>MVYKITVRVYQTNPDAFFHPVEKTVWKYANGGTWSITDDQHVLTMGGSGTSGTLRFHADNGESFTATFGVHNYKRWCDIVTNLAADETGMVINQQYYSQKNREEARERQLSNYQVKNAKGRNFQIVYTEAEGNDLHANLIIG[2x]

Sclerotium rolfsii lectin (SRL) is a cell wall-associated developmental–stage specific lectin secreted from the soil–born pathogenic fungus. SRL displays a clear specificity for TF and its substituted glycan structures. In the current study we report two recombinant variants SSR1 and SSR2, generated by the deliberate changes of the amino acids incorporated at particular sites of SRL by the synthetic gene construct method based on the complete amino acid sequence of SRL. Interestingly, SSR1 and SSR2 the two different variants of SRL, differ in their glycan specificity.

In case of SSR2 amino acids at the 1st, 14th, 34th, 113th and 123rd were replaced with Val, Asp, Ser, Gln and Gln, respectively. The crystal structures of SSR1 and SSR2 lectins in their free form were determined at 1.7 Å and 1.6 Å resolution, respectively. Like SRL there are two protein molecules (named mol A and mol B) in the crystallographic asymmetric unit of both variants related by a non-crystallographic two-fold symmetry. The mutations of SSR1 (N14D, E113Q, E123Q) and SSR2 (T1V, N14D, T34S, E113Q, E123Q) were all identified and all atoms of the mutated residues were well defined within the electron density map. A bound MPD molecule was found in both variants at the same place like in SRL while in the SSR2 structure two additional molecules form the crystallization medium were found bound (MPD and a 2-amino-2-hydroxymethyl-propane-1,3 diol). In the structure of SSR2 the mutated residues Val1 and Ser34 are located in strands S1 and S2, respectively. In the SSR2 structure the T1V mutation leads to a shift of the residue by 0.6–1.0 Å (depending on the atoms) while the T34S mutation does not cause any conformational change on this residue. The adoption of this conformation of Asn81 in SSR1 is made possible by a shift of the entire loop encompassing residues 81–86 by 3.0 Å on average, from their positions in the SRL structure. This shift is less profound in the SSR2 structure (1.0 Å on average) and does not lead to a change in the conformation of the side chain of Asn81 which maintains a similar conformation to that of the SRL structure. The carbohydrate binding property of SSR2 remains unaltered compared to SRL.> SNAPRGCDILIVYSPDAEEWCQYLQTLFLSSRQVRSQKILTHRLGPEASFSAEDLSLFLSTRCVVVLLSAELVQHFHKPSLLPLLQRAFHPPHRVVRLLCGVRDSEEFLDFFPDWAHWQELTCDDEPETYVAAVKKAIS

One such adaptor, B-cell adaptor for phosphoinositide 3-kinase (BCAP),4 functions in linking the B-cell receptor (BCR) and the co-receptor CD19 to the activation of PI3K via interaction with the SH2 domains on the regulatory p85 subunit. Architecturally, BCAP contains well defined ankyrin repeats and a Dof/BANK/BCAP (DBB) domain; the latter was first reported in the Drosophila protein Dof, where it is required for FGF-dependent signaling, and a homologous domain exists in the B-cell scaffold with ankyrin repeat (BANK) protein. A recent study predicted the existence of a TIR domain in the N-terminal region of BCAPL that is required for negative regulation of inflammatory signaling by TLRs. Here we present the structure of the N-terminal domain of BCAP, firmly establishing it as a TIR domain.

The N-terminal domain of BCAP comprising residues 7–142 was solubly expressed in Escherichia coli. The structure was solved at 2.5 Å using data derived from protein crystals in which the lysine residues were dimethylated and single-wavelength anomalous dispersion phasing with 5-amino-2,4,6-triiodoisophthalic acid monohydrate. There was a single molecule in the asymmetric unit, and the structure reveals that the N-terminal region adopts a typical TIR domain fold. The TIR domain of BCAP is composed of five parallel β-strands (βA–βE) surrounded by five α-helices(αA–αE). The third α-helix has a kink and forms two helices, αC and αC′, and the fourth is distorted. The loop regions, with the exception of the biologically important BB-loop, which connects the βB-strand to the αB-helix, were well defined in the electron density, and unlike the structure of the MAL-TIR domain, there are no disulfide bonds. Strikingly, the orientation of the βB-sheet and the αB-helix of BCAP TIR domain is such that it extends out of the domain core in comparison with that of MAL/TIRAP. The electrostatic potential of the solvent-accessible surface of BCAP reveals distinct regions of negative and positive potential in addition to hydrophobic patches, suggesting that the TIR domain of BCAP may interact with diverse TIR domain-containing proteins. The isolated TIR domain of BCAP is monomeric both in the crystal and in solution, a feature shared with most non-plant TIR domains, suggesting that vertebrate TIR domain-containing proteins require other domains to promote self-oligomerization: leucine-rich repeats (LRRs) for the TLR, a death domain for MyD88, and the DBB domain and likely the ANK repeats for BCAP.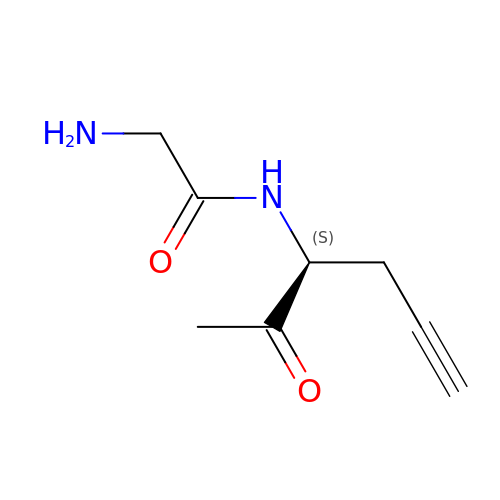2-azanyl-~{N}-[(3~{S})-2-oxidanylidenehex-5-yn-3-yl]ethanamide | C8 H12 N2 O2 | YHGRTOPUPRQLPX-ZETCQYMHSA-N6-PIPERIDIN-1-YLPYRIMIDINE-2,4-DIAMINE 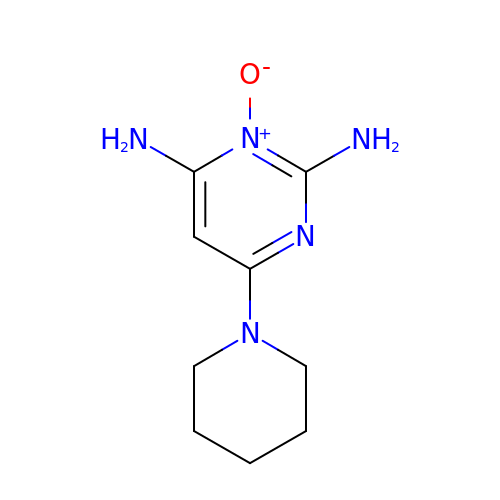3-OXIDE | C9 H15 N5 O | ZFMITUMMTDLWHR-UHFFFAOYSA-N>SNAMDIVSVALQRYSTKAFDPSKKLTAEEADKIKTLLQYSPSSTNSQPWHFIVASTEEGKARVAKSAAGNYTFNERKMLDASHVVVFCAKTAMDDAWLERVVDQEDADGRFATPEAKAANDKGRRFFADMHR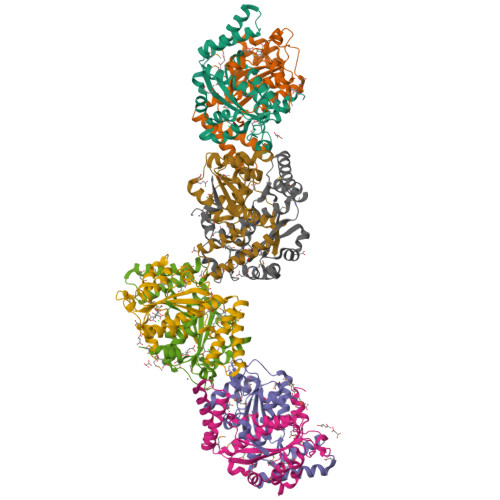VSLKDDHQWMAKQVYLNVGNFLLGVAAMGLDAVPIEGFDAEVLDAEFGLKEKGYTSLVVVPVGHHSVEDFNAGLPKSRLPLETTLTEV[8x]>[3x]MAGAIENARKEIKRISLEDHAESEYGAIYSVSGPVVIAENMIGCAMYELVKVGHDNLVGEVIRIDGDKATIQVYEETAGLTVGDPVLRTGKPLSVELGPGLMETIYDGIQRPLKAIKEESQSIYIPRGIDTPALDRTIKWQFTPGKFQVGDHISGGDIYGSVFENSLISSHKILLPPRSRGTITWIAPAGEYTLDEKILEVEFDGKKSDFTLYHTWPVRVPRPVTEKLSADYPLLTGQRVLDALFPCVQGGTTCIPGAFGCGKTVISQSLSKYSNSDAIIYVGCGERGNEMAEVLMEFPEL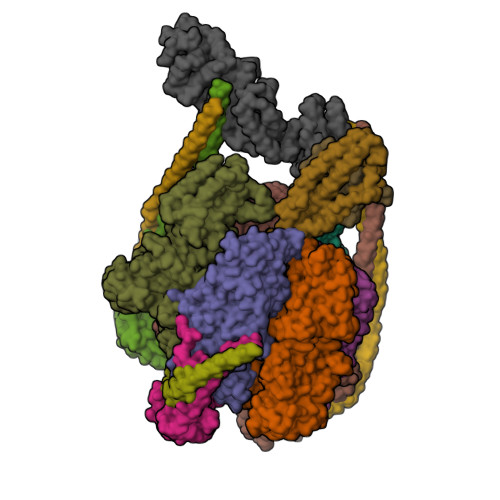YTEMSGTKEPIMKRTTLVANTSNMPVAAREASIYTGITLAEYFRDQGKNVSMIADSSSRWAEALREISGRLGEMPADQGFPAYLGAKLASFYERAGKAVALGSPDRTGSVSIVAAVSPAGGDFSDPVTTATLGITQVFWGLDKKLAQRKHFPSINTSVSYSKYTNVLNKFYDSNYPEFPVLRDRMKEILSNAEELEQVVQLVGKSALSDSDKITLDVATLIKEDFLQQNGYSTYDAFCPIWKTFDMMRAFISYHDEAQKAVANGANWSKLADSTGDVKHAVSSSKFFEPSRGEKEVHGEFEKLLSTMQERFAESTDDYKDHDGDYKDHDIDYKDDDDK;>MVLSDKELFAINKKAVEQGFNVKPRLNYNTVSGVNGPLVILEKVKFPRYNEIVNLTLPDGTVRQGQVLEIRGDRAIVQVFEGTSGIDVKKTTVEFTGESLRIPVSEDMLGRIFDGSGRPIDNGPKVFAEDYLDINGSPINPYARIYPEEMISTGVSAIDTMNSIARGQKIPIFSASGLPHNEIAAQICRQAGLVRPTKDVHDGHEENFSIVFAAMGVNLETARFFKQDFEENGSLERTSLFLNLANDPTIERIITPRLALTTAEYLAYQTERHVLTILTDMSSYADALREVSAAREEVPGRRGYPGYMYTDLSTIYERAGRVEGRNGSITQIPILTMPNDDITHPIPDLTGYITEGQIFVDRQLHNKGIYPPINVLPSLSRLMKSAIGEGMTRKDHGDVSNQLYAKYAIGKDAAAMKAVVGEEALSIEDKLSLEFLEKFEKTFITQGAYEDRTVFESLDQAWSLLRIYPKEMLNRISPKILDEFYDRARDDADEDEEDPDTRSSGKKKDASQEESLI[3x];>MSSAITALTPNQVNDELNKMQAFIRKEAEEKAKEIQLKADQEYEIEKTNIVRNETNNIDGNFKSKLKKAMLSQQITKSTIANKMRLKVLSAREQSLDGIFEETKEKLSGIANNRDEYKPILQSLIVEALLKLLEPKAIVKALERDVDLIESMKDDIMREYGEKAQRAPLEEIVISNDYLNKDLVSGGVVVSNASDKIEINNTLEERLKLLSEEALPAIRLELYGPSKTRKFFD[3x];>[3x]MSQKNGIATLLQAEKEAHEIVSKARKYRQDKLKQAKTDAAKEIDSYKIQKDKELKEFEQKNAGGVGELEKKAEAGVQGELAEIKKIAEKKKDDVVKILIETVIKPSAEVHINAL;> MSGNREQVFPTRMTLGLMKTKLKGANQGYSLLKRKSEALTKRFRDITKRIDDAKQKMGRVMQTAAFSLAEVSYATGENIGYQVQESVSTARFKVRARQENVSGVYLSQFESYIDPEINDFRLTGLGRGGQQVQRAKEIYSRAVETLVELASLQTAFIILDEVIKVTNRRVNAIEHVIIPRTENTIAYINSELDELDREEFYRLKKVQEKKQNETAKLDAEMKLKRDRAEQDASEVAADEEPQGETLVADQEDDVIF;> MAEKRTLIAVIADEDTTTGLLLAGIGQITPETQEKNFFVYQEGKTTKEEITDKFNHFTEERDDIAILLINQHIAENIRARVDSFTNAFPAILEIPSKDHPYDPEKDSVLKRVRKLFGE;> MGATKILMDSTHFNEIRSIIRSRSVAWDALARSEELSEIDASTAKALESILVKKNIGDGLSSSNNAHSGFKVNGKTLIPLIHLLSTSDNEDCKKSVQNLIAELLSSDKYGDDTVKFFQEDPKQLEQLFDVSLKGDFQTVLISGFNVVSLLVQNGLHNVKLVEKLLKNNNLINILQNIEQMDTCYVCIRLLQELAVIPEYRDVIWLHEKKFMPTLFKILQRATDSQLATRIVATNSNHLGIQLQYHSLLLIWLLTFNPVFANELVQKYLSDFLDLLKLVKITIKEKVSRLCISIILQCCSTRVKQHKKVIKQLLLLGNALPTVQSLSERKYSDEELRQDISNLKEILENEYQELTSFDEYVAELDSKLLCWSPPHVDNGFWSDNIDEFKKDNYKIFRQLIELLQAKVRNGDVNAKQEKIIIQVALNDITHVVELLPESIDVLDKTGGKADIMELLNHSDSRVKYEALKATQAIIGYTFK>MTPDELNSAVVTFMANLNIDDSKANETASTVTDSIVHRSIKLLEVVVALKDYFLSENEVERKKALTCLTTILAKTPKDHLSKNECSVIFQFYQSKLDDQALAKEVLEGFAALAPMKYVSINEIAQLLRLLLDNYQQGQHLASTRLWPFKILRKIFDRFFVNGSSTEQVKRINDLFIETFLHVANGEKDPRNLLLSFALNKSITSSLQNVENFKEDLFDVLFCYFPITFKPPKHDPYKISNQDLKTALRSAITATPLFA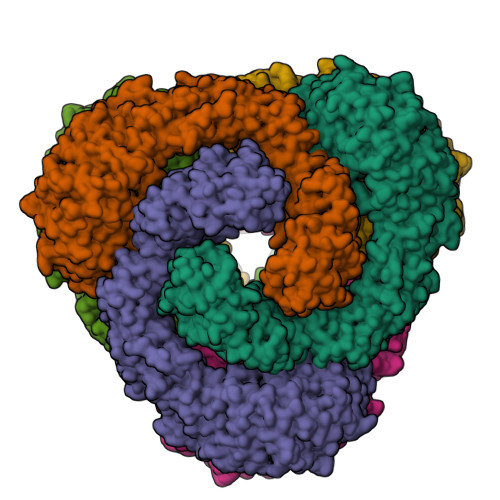EDAYSNLLDKLTASSPVVKNDTLLTLLECVRKFGGSSILENWTLLWNALKFEIMQNSEGNENTLLNPYNKDQQSDDVGQYTNYDACLKIINLMALQLYNFDKVSFEKFFTHVLDELKPNFKYEKDLKQTCQILSAIGSGNVEIFNKVISSTFPLFLINTSEVAKLKLLIMNFSFFVDSYIDLFGRTSKESLGTPVPNNKMAEYKDEIIMILSMALTRSSKAEVTIRTLSVIQFTKMIKMKGFLTPEEVSLIIQYFTEEILTDNNKNIYYACLEGLKTISEIYEDLVFEISLKKLLDLLPDCFEEKIRVNDEENIHIETILKIILDFTTSRHILVKESITFLATKLNRVAKISKSREYCFLLISTIYSLFNNNNQNENVLNEEDALALKNAIEPKLFEIITQESAIVSDNYNLTLLSNVLFFTNLKIPQAAHQEELDRYNELFISEGKIRILDTPNVLAISYAKILSALNKNCQFPQKFTVLFGTVQLLKKHAPRMTETEKLGYLELLLVLSNKFVSEKDVIGLFDWKDLSVINLEVMVWLTKGLIMQNSLESSEIAKKFIDLLSNEEIGSLVSKLFEVFVMDISSLKKFKGISWNNNVKILYKQKFFGDIFQTLVSNYKNTVDMTIKCNYLTALSLVLKHTPSQSVGPFINDLFPLLLQALDMPDPEVRVSALETLKDTTDKHHTLITEHVSTIVPLLLSLSLPHKYNSVSVRLIALQLLEMITTVVPLNYCLSYQDDVLSALIPVLSDKKRIIRKQCVDTRQVYYELGQIPFE[6x]ABCG2 transports uric acid and plays an essential role in the pathology of gout, but also confers resistance to a variety of chemotherapeutics including topoisomerase inhibitors (i.e., mitoxantrone (MXN), etoposide, topotecan, SN38), anthracyclines (i.e., doxorubicin and daunorubicin), antimetabolites (i.e., methotrexate and 5-fluorouracil), and photosensitizers (i.e., pheophorbide A). There are more than 200 known ABCG2 substrates which have highly diverse chemical structures and functions, and the substrate spectrum of ABCG2 is substantially overlapping with and yet distinct from that of Pgp or ABCC14. In this work, we used cryo-EM and biochemical assays to characterize the structures of ABCG2 in the unliganded state, and in the presence of the chemotherapeutic agents imatinib, MXN, or SN38. In total, our results delineate a new paradigm for the conformational transition cycle of ABCG2, and reveal how different chemotherapy compounds distinctively alter the conformational space of the transporter.

We subjected purified and nanodisc reconstituted human ABCG2 to single-particle cryo-EM analysis in the absence of antibody fragments or bound ligands. In the apo state, ABCG2 adopted a single predominant conformation that was distinct from that seen previously with the Fab or ligand bound transporter. In the absence of 5D3 fab or bound ligands the TM helices adopt a closed conformation while the NBDs remain separate in a nucleotide-free state. In the apo-closed conformation the TM helices form a tightly packed helical bundle near the cytosolic region, primarily as a result of the intracellular region of TM5 residing closer to TM1 and TM2 of the opposite ABCG2 monomer. In the apo-closed conformation the position of TM5 seals the crevice between ABCG2 monomers where substrates and inhibitors bound in the previous inward facing structures. However, in our apo-closed conformation TM5 is also rotated nearly 180° along the helical axis, thus generating an entirely different overall protein conformation. However, the helical rotation of TM5 observed in our apo-closed structure causes the Phe545 sidechain to face the opposite ABCG2 monomer. In the apo-closed conformation the positioning of TM5 results in these sidechains being oriented towards the dimer interface, such that a sulfur cluster of 10 cysteines and methionines along TM5 and TM2 is formed at the central 2-fold axis between ABCG2 monomers. Whereas the middle portion of TM2 (residues 434–438) adopts a helical character in the previous inward facing and ATP bound structures, this stretch of helix unwinds and bows outwards towards the lateral sides of the transporter in our apo-closed structure. However, as a result of the helical unraveling of TM2 observed in our apo-closed structure the Phe439 phenyl moiety is flipped ~180° outward and away from the 2-fold axis.

>MSSSNVEVFIPVSQGNTNGFPATASNDLKAFTEGAVLSFHNICYRVKLKSGFLPCRKPVEKEILSNINGIMKPGLNAILGPTGGGKSSLLDVLAARKDPSGLSGDVLINGAPRPANFKCNSGYVVQDDVVMGTLTVRENLQFSAALRLATTMTNHEKNERINRVIQELGLDKVADSKVGTQFIRGVSGGERKRTSIGMELITDPSILFLDEPTTGLDSSTANAVLLLLKRMSKQGRTIIFSIHQPRYSIFKLFDSLTLLASGRLMFHGPAQEALGYFESAGYHCEAYNNPADFFLDIINGDSTAVALNREEDFKATEIIEPSKQDKPLIEKLAEIYVNSSFYKETKAELHQLSGGEKKKKITVFKEISYTTSFCHQLRWVSKRSFKNLLGNPQASIAQIIVTVVLGLVIGAIYFGLKNDSTGIQNRAGVLFFLTTNQCFSSVSAVELFVVEKKLFIHEYISGYYRVSSYFLGKLLSDLLPMRMLPSIIFTCIVYFMLGLKPKADAFFVMMFTLMMVAYSASSMALAIAAGQSVVSVATLLMTICFVFMMIFSGLLVNLTTIASWLSWLQYFSIPRYGFTALQHNEFLGQNFCPGLNATGNNPCNYATCTGEEYLVKQGIDLSPWGLWKNHVALACMIVIFLTIAYLKLLFLKKYS[2x]> GSHMEELQNKLEDVVIDRNLLILGKILGEGEFGSVMEGNLKQEDGTSLKVAVKTMKLDNSSQREIEEFLSEAACMKDFSHPNVIRLLGVCIEGIPKPMVILPFMKYGDLHTYLLYSRLETGPKHIPLQTLLKFMVDIALGMEYLSNRNFLHRDLAARNCMLRDDMTVCVADFGLSKKIYSGDYYRQGRIAKMPVKWIAIESLADRVYTSKSDVWAFGVTMWEIATRGMTPYPGVQNHEMYDYLLHGHRLKQPEDCLDELYEIMYSC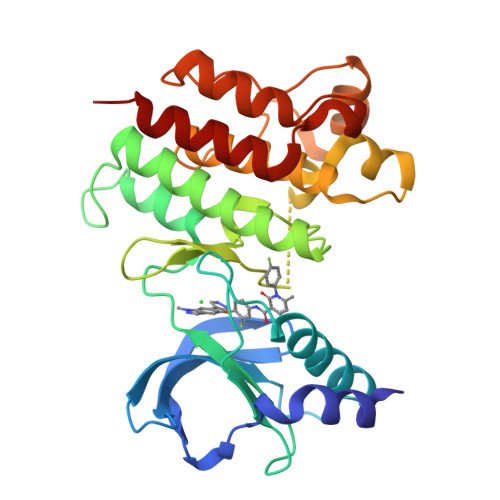WRTDPLDRPTFSVLRLQLEKLLESLPDV>GAMG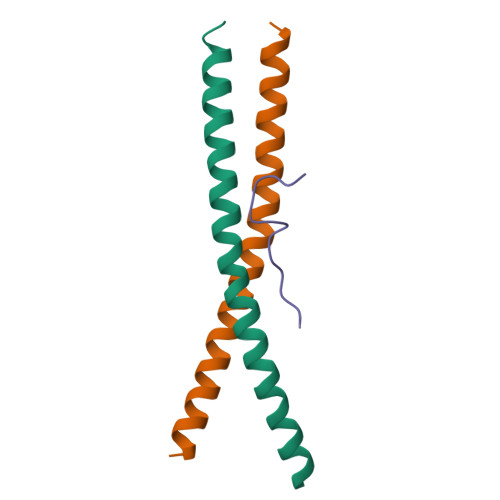SFNSSINNIHEMEIQLKDALEKNQQWLVYDQQREVYVKGLLAKIFELEKKTETAAHSLP[8x];>[4x]DLAVGPPSLNYPGY> MANVPWAEVCEKFQAALALSRVELHKNPEKEPYKSKYSARALLEEVKALLGPAPEDEDERPEAEDGPGAGDHALGLPAEVVEPEGPVAQRAVRLAVIEFHLGVNHIDTEELSAGEEHLVKCLRLLRRYRLSHDCISLCIQAQNNLGILWSEREEIETAQAYLESSEALYNQYMKEVGSPPLDPTERFLPEEEKLTEQERSKRFEKVYTHNLYYLAQVYQHLEMFEKAAHYCHSTLKRQLEHNAYHPIEWAINAATLSQFYINKLCFMEARHCLSAANVIFGQTGKISATEDTPEAEGEVPELYHQRKGEIARCWIKYCLTLMQNAQLSMQDNIGELDLDKQSELRALRKKELDEEESIRKKAVQFGTGELCDAISAVEEKVSYLRPLDFEEARELFLLGQHYVFEAKEFFQIDGYVTDHIEVVQDHSALFKVLAFFETDMERRCKMHKRRIAMLEPLTVDLNPQYYLLVNRQIQFEIAHAYYDMMDLKVAIADRLRDPDSHIVKKINNLNKSALKYYQLFLDSLRDPNKVFPEHIGEDVLRPAMLAKFRVARLYGKIITADPKKELENLATSLEHYKFIVDYCEKHPEAAQEIEVELELSKEMVSLLPTKMERFRTKMALT

Kinesin-binding protein (KIFBP), which is mutated in Goldberg-Shprintzen syndrome, binds to and inhibits the catalytic motor heads of 8 of 45 kinesin superfamily members, but the mechanism remains poorly defined. KIFBP interacts directly with the motor head of Kinesin-2 (KIF3A), Kinesin-3 (KIF1A, KIF1B, KIF1C, KIF13B, and KIF14), Kinesin-8 (KIF18A), and Kinesin-12 (KIF15) family members, resulting in inhibition of motor-microtubule binding both in vitro and in cells. We show that KIFBP is a tandem repeat protein constructed of nine helix pairs that assemble into a solenoid-like structure. Collectively, our work describes the molecular mechanism of KIFBP-mediated inhibition of KIF15 and KIF18A via binding to and stabilizing a conformation of the kinesin motor head that is incompatible with microtubule binding.

To determine an atomic model of KIFBP, we used cryo-EM to determine the overall structure of KIFBP and a higher-resolution structure of the N terminus of KIFBP. Given that the resolution of 4.6 Å is not sufficient to build an atomic model, we wanted to improve the resolution of our reconstruction. To this end, we performed masking and three-dimensional (3D) classification on the N-terminal two-thirds of KIFBP to obtain a higher-resolution structure at 3.8 Å. Our atomic model provides a high-confidence positioning of KIFBP residues, allowing us to map the structure onto the KIFBP sequence, confirming α-helical positions, and showing the locations of loops connecting HPs throughout the structure. We determined a near-atomic structure of KIFBP corresponding to ~40 of 72 kDa, using this reconstruction for de novo model building. This places the KIFBP reconstruction and model among the smallest–molecular weight macromolecules to be built de novo by cryo-EM. The relatively small size of KIFBP may be the driving factor limiting the overall resolution of KIFBP alone to ~3.8 Å instead of obtaining higher-resolution reconstructions.2-HYDROXY-4,5-DIOXOHEPTYL HYDROGEN PHOSPHONATE | C7 H13 O6 P | 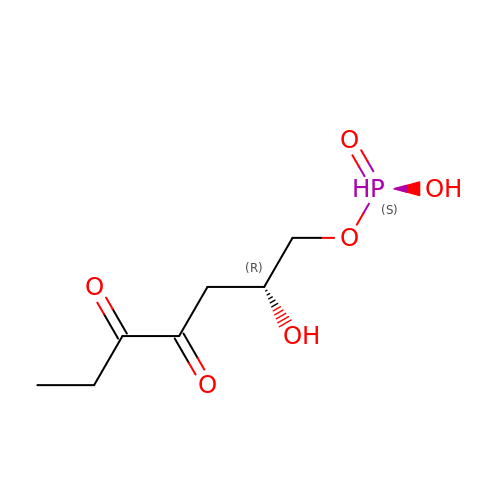PYYIHKXJWNSAKF-RXMQYKEDSA-N Cilia and flagella associated protein 410 (CFAP410) is a protein localized at the basal body of cilia/flagella and plays essential roles in ciliogenesis. Our work revealed that CFAP410 is a bimodular protein comprising two highly conserved domains, including a leucine rich repeat (LRR) motif at its N-terminus and an oligomeric helical bundle at its C-terminus. CFAP410 was shown to localize to the basal body and interacts with NEK1 and SPATA7 during ciliogenesis and DNA damage repair. Homo sapiens CFAP410 (HsCFAP410, accession code: NP_004919) is 256 amino acids long and a number of single residue mutations, including I35F, C61Y, R73P, Y107C, Y107H, V111M and L224P, have been associated with skeletal and/or retinal disorders.

Here we report a 1.0-Å resolution crystal structure of the N-terminal domain (NTD) of Trypanosoma brucei CFAP410. In the end we obtained crystals only for the construct spanning residues 1–160, which is what NTD refers to in all subsequent structural analyses of TbCFAP410. Residues 1–138 fold into a canonical leucine-rich repeat (LRR), with five tandem repeats forming a calzone-like structure. The LRR motif contains five parallelly arranged β strands forming a flat sheet on one side and an array of four short α helices on the other. The space between the α helices and the β strands constitutes the hydrophobic core of the LRR motif and is packed with many highly conserved leucine residues. Additionally, we found that residues 139–160 of TbCFAP410 forms a long hairpin-like loop, which is tightly packed on top of the helical surface of the LRR motif. The loop makes extensive contacts with the LRR motif via six hydrogen bonds and numerous hydrophobic interactions. All TbCFAP410 truncations with the intact loop were soluble, whereas those lacking parts or the whole loop, i.e., constructs covering residues 1–149 and 1–140, were all insoluble upon expression in E. coli. This further suggests that the loop is essential to facilitate the folding and/or to stablize the structure of the LRR motif in TbCFAP410. In the crystal structure of TbCFAP410-NTD there is an extensive surface patch across all five strands of the β sheet. Location of individual residues corresponding to the five disease-causing mutations in HsCFAP410 can be clearly visualized in TbCFAP410. These residues can be grouped into three categories, including one surface residue that is fully exposed to solvent (R75), two semi-exposed residues (V37 and Y107), and two hidden residues that are completely buried in the hydrophobic core of the structure (C63 and V111).

> GHMAGVLTENLVLQKTKVDSIQRVRKLNVCAAQLSDIGVLRRACNLEVLSLSLNELSELGVLENCPRLSELYLRKNRVEDLNQVLHLSDAPNLTVLTLTENPICQDPNYRRFVIAAVGSLQRLDDIDILPQEREEAYRVFPNLHAIAPPPSLYCDPAKGKIR> GGGMKTKQGVHVHNLVFETILGIL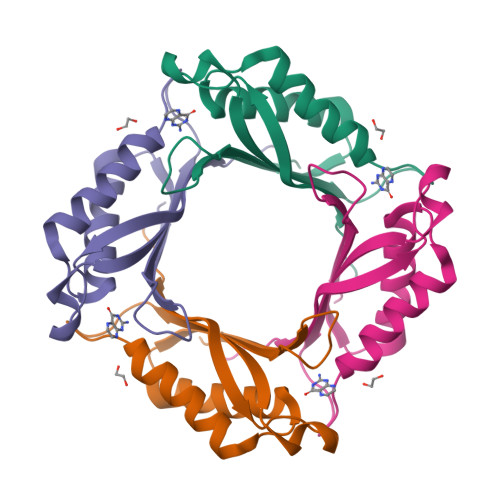EFERLKPQKISVDLDLFYTQLPNKAYLDYIKIQELIQKMMQEKQYLLIEDALKDLSQILKTRYKEITELYLKISKLEISPDSQVGASVKICYENNL>[2x]RMEIVKIPVVVHVVWNEEEENISDAQIQSQIDILNKDFRKLNSDVSQVPSVWSNLIADLGIEFFLATKDPNGNQTTGITRTQTSVTFFTTSDEVKFASSGGEDAWPADRYLNIWVCHVLKSEIGQDILGYAQFPGGPAETDGVVIVDAAFGTTGTALPPFDKGRTATHEIGHWLNLYHIWGDELRFEDPCSRSDEVDDTPNQADPNFGAPSYPHVSCSNGPNGDMFMNYMDYVDDKCMVMFTQGQATRVN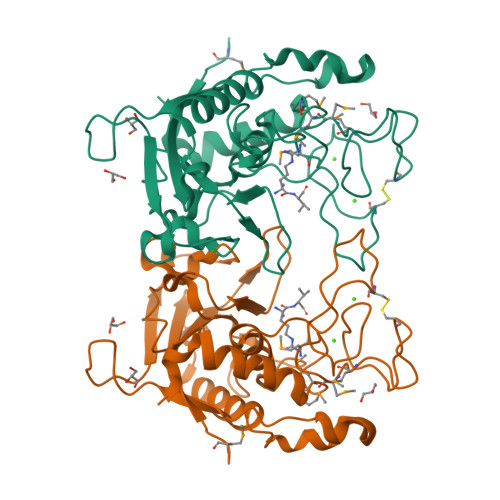ACLDGPRSSFLA>LQFHAFISYSEHDSAWVKSELVPYLEKEDIQICLHERNFVPGKSIVENIINCIEKSYKSIFVLSPNFVQSEWCHYELYFAHHNLFHEGSNNLILILLEPIPQNSIPNKYHKLKALMTQRTYLQWPKEKSKRGLFWANIRAAFNMKLTLVTENNDVKSMKLTLVTENNDVKSLE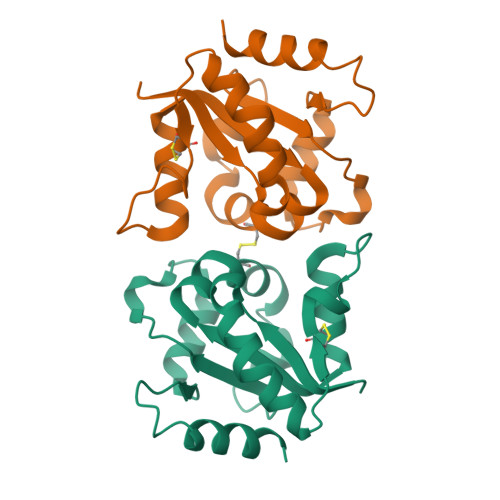HHHHHH[2x]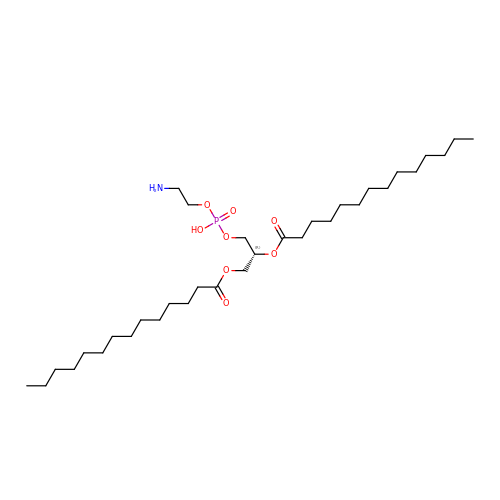(2R)-3-{[(S)-(2-aminoethoxy)(hydroxy)phosphoryl]oxy}-2-(tetradecanoyloxy)propyl tetradecanoate | C33 H66 N O8 P | NEZDNQCXEZDCBI-WJOKGBTCSA-N>[2x]MSTPGAQQVLFRTG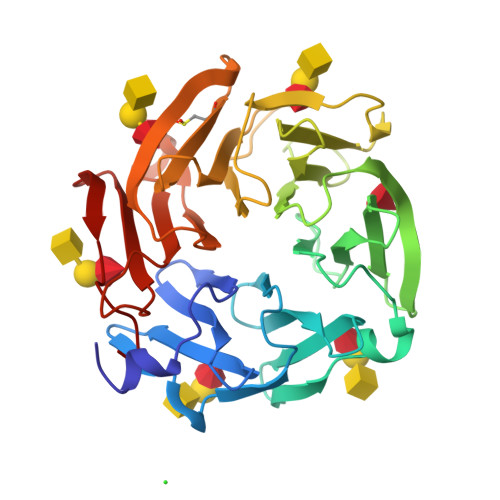IAAVNSTNHLRVYFQDVYGSIRESLYEGSWANGTEKNVIGNAKLGSPVAATSKELKHIRVYTLTEGNTLQEFAYDSGTGWYNGGLGGAKFQVAPYSCIAAVFLAGTDALQLRIYAQKPDNTIQEYMWNGDGWKEGTNLGGALPGTGIGATSFRYTDYNGPSIRIWFQTDDLKLVQRAYDPHKGWYPDLVTIFDRAPPRTAIAATSFGAGNSSIYMRIYFVNSDNTIWQVCWDHGKGYHDKGTITPVIQGSEVAIISWGSFANNGPDLRLYFQNGTYISAVSEWVWNRAHGSQLGRSALPPA C. neoformans sterylglucosidase 1 (Sgl1), the first gene/protein identified with a sterylglucosidase activity, converts erg-glc to ergosterol and glucose. Our analysis of structures of C. neoformans Sgl1 reveals a Y-shaped hydrophobic active site pocket that generates specificity for erg-glc and which is not present in human and bacterial glucosylceramidases. Sgl1 is an ideal pharmacological target with broad spectrum since Sgl1 is widely conserved in fungi and there is no obvious homolog in humans.

Screening of three deletion constructs identified one deletion, C. neoformans Sgl1 Δ723–777, that did not affect Sgl1 activity towards erg-glc and yielded crystals that diffracted to 2.1 Å resolution. The deleted region between residues 723 and 777 is not conserved among Sgl1 orthologs and appears specific for C. neoformans Sgl1 with no obvious role in Sgl1 function or regulation. The structure of Sgl1 revealed two domains comprising a catalytic domain with a central TIM barrel and a C-terminal β-sandwich domain. The main differences resided in the larger catalytic domain of Sgl1 that contains 10 β-strands, 28 α-helices, and several ordered loops. These additional structural elements combine to form a unique cap region above the TIM barrel that creates an enclosed Y-shaped cavity. The active site of Sgl1 is located at the base of the Y-shaped cavity and is capped to limit binding to a single glucose moiety. One arm of the Y-shaped cavity is lined with hydrophobic residues and is buried within the protein structure, which would limit the size of molecules that can fit in this cavity. The other arm is also lined with hydrophobic residues and contains a narrow opening that is solvent-exposed. The active site of Sgl1 contained two catalytic glutamate residues found in the canonical topological positions for retaining β-glucosidases. However, unlike EGCase II, Sgl1 contained a series of capping residues, including a bulky Trp residue that creates a wall to sterically hinder substrates with more than one sugar from binding. The unique active sites of Sgl1 and Cerezyme suggest that selective inhibitors targeting Sgl1 would not inhibit Cerezyme. In support of this, binding of a Tris molecule in the active site of Sgl1 resulted in the Tris molecule adopting a different conformation than that of a Tris molecule previously observed in the active site of Cerezyme13.

>[4x]SMPPPPEVSPVTGNPVSPHYIHSSTLHFQDVNGRSLVLRGVNLSGSAKHPNNQPSHIREGFWETAEAGKGDFINKPLNLDDGSADLHLARLKAWGYNLLRYVFTWESLEHAGPKEYDYAYMDYIIAVLRKCKEWGFRVFMDPHQDVWSRFTGGSGAPLWTLYACGIDPYHLTATAAAYLHCEWPSAESPKPQDFPAMIWGTNYTHLANQTIWTFFFAGKTYAPKCIIDGKNIQDFLQDHFIDAVGELAKRIAEEAGDLLDECVIGWDSINEPGEGLIGCKDLAVIPAEQQLKKGPSPTPIEGMRLGMGEAQDVQAWNFGPMGPYRGSRQTIDPKGVKLWLSKEDDVKRGSGKWGWTRGKEWALGTCIWAHHGVWEIATSTLLRPDYFSTLPTNPGHQVDFVDDFWALHWLAYSSRIRLHHPESIHFIQAPVLRQPPKLPESFLKGRACSSPHFYDGLTLMTKHWNWFNADAIGVIRKKYWSIVQAVRIGEGPIRKMIQGELAVLKQDTIDILGNYPTLVGEIGIPYDMDDKKAYGYVDGGRGEGDYSSQQKAMDCSMNACDGPNCLNYAIWNYVPDNVHEWGDNWNGEDLSLWSVDDKEQESYHDSPRSDTPNFSTNSNSLTNSSATLTVPMSGASKLRPSPSVIDSGDFSPTLILDGSRAVAAFCRPYPVATVGIPERIDFDITSTKFKYAVRVRADDIANEQVYTEIYLPFVHYAASLNASYSSFAQLSLDVTIVASHGRVEIQGQTLRWWYPVPGTGEEVYTIEVQRNGGALRRDLGYVQQGNFLDVCPECVIA> 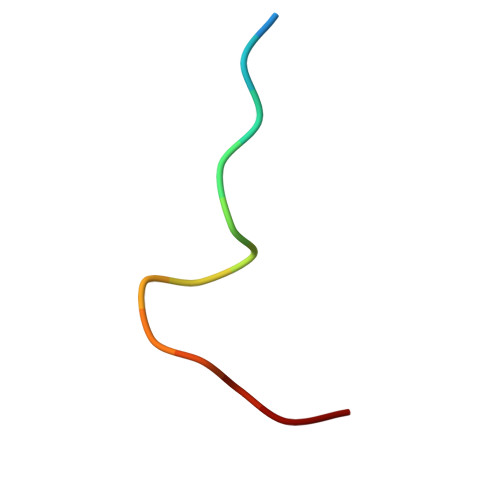DLAVGPPSLNYIPP> ASMKQPVVVIGSGLAGLTTSNRLISKYRIPVVLLDKAASIGGNSIKASSGINGAHTDTQQNLKVMDTPELFLKDTLHSAKGRGVPSLMDKLTKESKSAIRWLQTEFDLKLDLLAQLGGHSVPRTHRSSGKLPPGFEIVQALSKKLKDISSKDSNLVQIMLNSEVVDIELDNQGHVTGVVYMDENGNRKIMKSHHVVFCSGG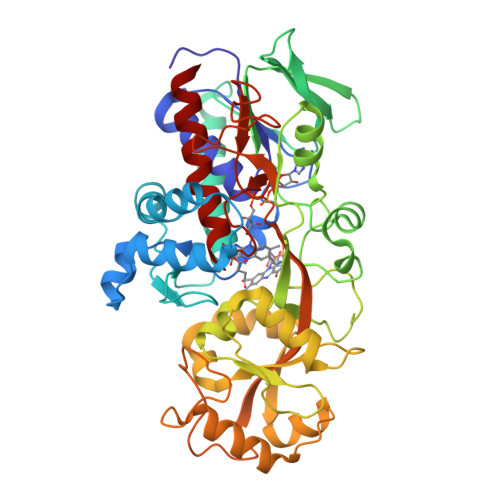FGYSKEMLKEYSPNLIHLPTTNGKQTTGDGQKILSKLGAELIDMDQVQVHPTGFIDPNDRENNWKFLAAEALRGLGGILLHPTTGRRFTNELSTRDTVTMEIQSKCPKNDNRALLVMSDKVYENYTNNINFYMSKNLIKKVSINDLIRQYDLQTTASELVTELKSYSDVNTKDTFDRPLIINAFDKDISTESTVYVGEVTPVVHFTMGGVKINEKSQVIKKNSESVLSNGIFAAGEVSGGVHGANRLGGSSLLECVVFGKTAADNIAKLY2-{[(S)-(2-aminoethoxy)(hydroxy)phosphoryl]oxy}ethyl heptadecanoate | C21 H44 N O6 P | 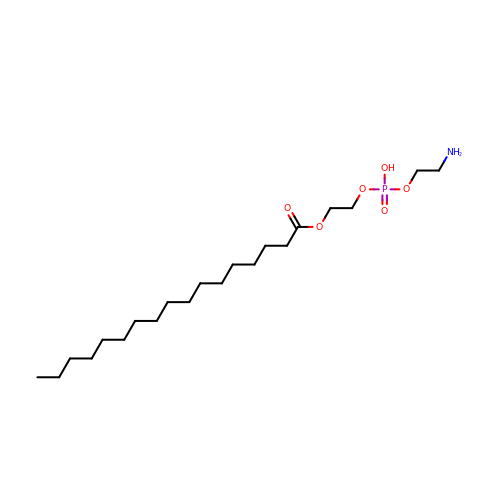KBKQEKNZSDBGFI-UHFFFAOYSA-N> NFTQTLQKDANASSEFYINKLGQTQELEDQQTYKLLAARVLIRENKVEQSAALLRELGELNDAQKLDRALIEARISAAKNANEVAQNQLRALDLNKLSPSQKSRYYETLAIVAENRKDMIEAVKARIEMDKNLTDVQRHQDNIDKTWALLRSANTGVINNASDEGNAALGGWLTLIKAYNDYIRQPVQLSQALQSWKNAYPNHAAATLFPKELLTLLNFQQTNVSQIGLLLPLSGDGQILGTTIQSGFNDAKGNSTIPVQVFDTSMNSVQDIIAQAKQAGIKTLVGPLLKQNLDVILADPAQIQGMDVLALNATPNSRAIPQLCYYGLSPEDEA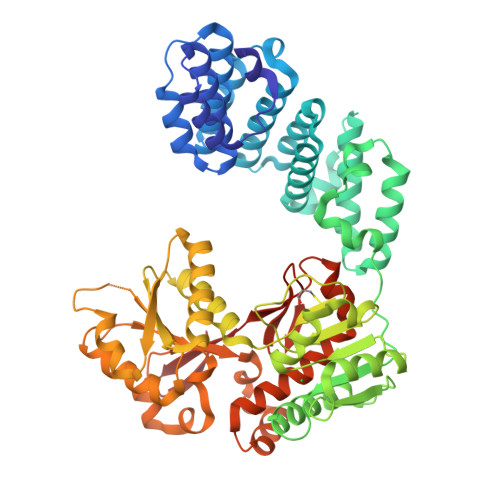ESAANKMWNDGVRNPLVAMPQNDLGQRVGNAFNVRWQQLAGTDANIRYYNLPADVTYFVQENNSNTTALYAVASPTELAEMKGYLTNIVPNLAIYASSRASASATNTNTDFIAQMNGVQFSDIPFFKDTNSPQYQKLAKSTGGEYQLMRLYAMGADAWLLINQFNELRQVPGYRLSGLTGILSADTNCNVERDMTWYQYQDGAIVPVAN>[4x]SEMTPREIVSELDKHIIGQDNAKRSVAIALRNRWRRMQLNEELRHEVTPKNILMIGPTGVGKTEIARRLAKLANAPFIKVEATKFTEVGYVGKEVDSIIRDLTDAAVKMVRVQAIEKNRYRAEELAEERILDVLIPPAKNNWGQTEQQQEPSAARQAFRKKLREGQLDDKEIEIDLAAAPMGVEIMAPPGMEEMTSQLQSMFQNLGGQKQKARKLKIKDA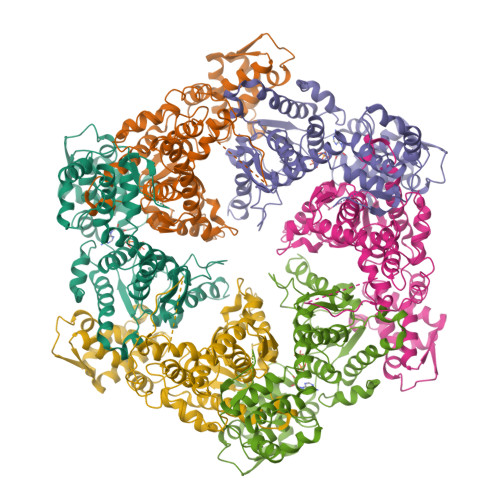MKLLIEEEAAKLVNPEELKQDAIDAVEQHGIVFIDEIDKICKRGESSGPDVSREGVQRDLLPLVEGCTVSTKHGMVKTDHILFIASGAFQIAKPSDLIPELQGRLPIRVELQALTTSDFERILTEPNASITVQYKALMATEGVNIEFTDSGIKRIAEAAWQVNESTENIGARRLHTVLERLMEEISYDASDLSGQNITIDADYVSKHLDALVADEDLSRFIL> AALPDQSFLWNVFQRVDKDRSGVISDTELQQALSNGTWTPFNPVTVRSIISMFDRENKAGVNFSEFTGVWKYITDWQNVFRTYDRDNSGMIDKNELKQALSGAGYRL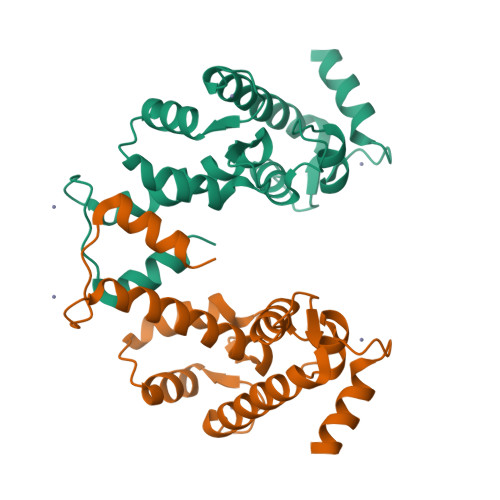SDQFHDILIRKFDRQGRGQIAFDDFIQGCIVLQRLTDIFRRYDTDQDGWIQVSYEQYLSMVFSIV> AQREKDTRISKKMETMGIYFATPEWVALNGHRGPSPGQLKYWQNTREIPDPNEDYLDYVHAEKSRLASEEQILRAATSIYGAPGQAEPPQAFIDEVAKVYEI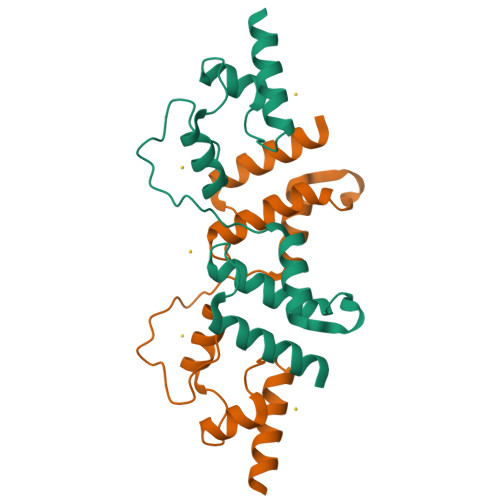NHGRGPNQEQMKDLLLTAMEMKH2-[[(1~{S},2~{S})-2-[methyl-[(6-methylpyridin-2-yl)methyl]amino]cyclohexyl]-[(6-methylpyridin-2-yl)methyl]amino]ethanoic acid | C23 H32 N4 O2 | 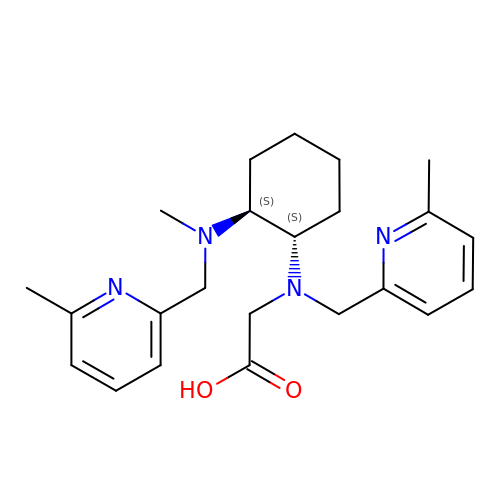SKWHQCFCFFYXHR-VXKWHMMOSA-N>MSPYSSDTTPCCFAYIARPLPRAHIKEYFYTSGKCSNPAVVFVTRKNRQVCANPEKKWVREYINSLSMS[2x];> MSPYSSDTTPCCFAYIARPLPRAHIKEYFYTSGKCSNPAVVFVTRK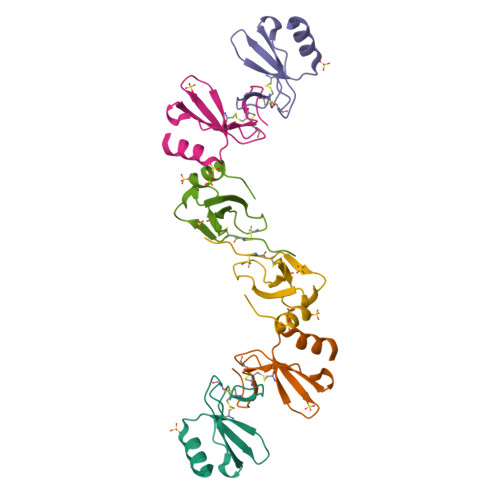NRQVCANPEKKWVREYINSLEMS>MRFVMPGDRIGSAEEYVKGEGVYEEGGELFAAVAGKL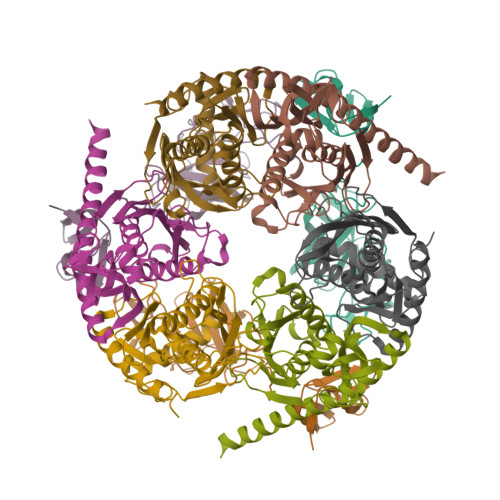IIKDRVAKVESISPIPEIVKGDVVLGRVVDLRNSIALIEVSSKKGENRGPSNRGIGILHVSNVDEGYVKEISEAVGYLDILKARVIGDNLRLSTKEEEMGVLRALCSNCKTEMVREGDILKCPECGRVEKRKISTDYGKGEW[3x];>[3x]MSEFNEKPEKLIVDGLRLDGRKFDELRPIKIEASVLKRADGSCYLEMGKNKVIAAVFGPREVHPRHLQDPSKAIIRYRYNMAPFSVEERKRPGPDRRSIEISKVSKEAFEAVIMKELFPRSAIDIFVEVLQADAGSRTACLNAASVALVDAGVPMKGMITSVAVGKADGQLVLDPMKEEDNFGEADMPFAFLIRNGKIESIALLQMDGRMTRDEVKQAIELAKKGALQIYEMQREAILRRYIEVGEEMDEITEGGEDA;>MPEDILVDIKRDYVLSKLRDNERIDGRGFDEFRKVEIIPNVIEKAEGSALVKLGDTQVVVGVKMQPGEPYPDTPDRGVIIVNAELVPLASPTFEPGPPDENSIELARVVDRGIRESEAVDLSKLVIEEGEKVWIVFVDIHALDDDGNLLDASALAAIAALMNTKVPAERFDLGEDYLLPVRDLPVSVTSLIVGNKYLVDPSREEMSVGDTTLTITTDKDDNVVAMQKSGGYLLDEKLFDELLDVSINCARKLREKFKEI[3x]> RSVYELDCIPLWGTVS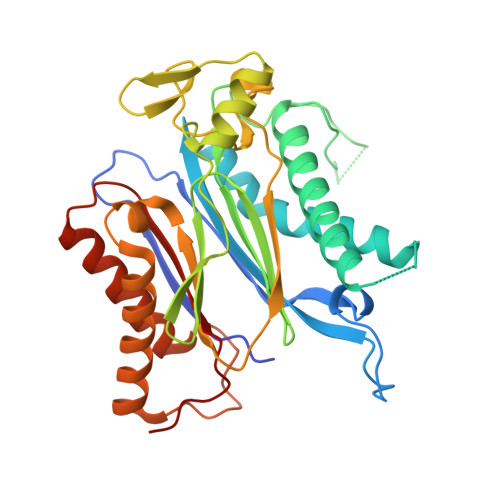IQGNRSEMEDAFAVSPHFLKLPIKMLMGDHEGESPSLTHLTGHFFGVYDGHGGHKVADYCRDRLHFALAEEIERIKDELCKRNTGEGRQVQWDKVFTSCFLTVDGEIEGKIGRAVVGSSDKVLEAVASETVGSTAVVALVCSSHIVVSNCGDSRAVLFRGKEAMPLSVDHKPDREDEYARIENAGGKVIQWQGARVFGVLAMSRSIGDRYLKPYVIPEPEVTFMPRSREDECLILASDGLWDVMNNQEVCEIARRRILMWHKKNGAPPLAERGKGIDPACQAAADYLSMLALQKGSKDNISIIVIDLKAQRKFKTRT> MVNMVSNPGFEDGLDSWQDWQQDMSAVPEAAHNGALGLKIGGGKAAGGGQDIPLKPNTTYILGAWAKFDSKPAGTFDVVVQYHLKDANNTYVQHILNFNETDWTYKQLLFTTPDVFGSTPELALWKGDTSKANLYVDDVY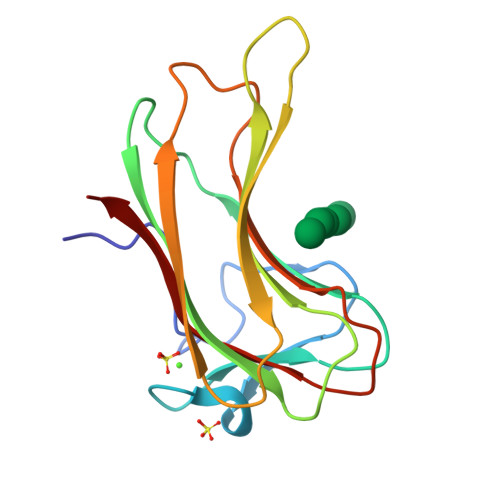LVEV> MASDYKDDDDKASDEVDAGTMANVSKKVSWSGRDRDDEEAAPLLRRTARPGGGTPLLNGAGPGAARQSPRSALFRVGHMSSVELDDELLDPDMDPPHPFPKEIPHNEKLLSLKYESLDYDNSENQLFLEEERRINHTAFRTVEIKRWVICALIGILTGLVACFIDIVVENLAGLKYRVIKGNIDKFTEKGGLSFSLLLWATLNAAFVLVGSVIVAFIEPVAAGSGIPQIKCFLNGVKIPHVVRLKTLVIKVSGVILSVVGGLAVGKEGPMIHSGSVIAAGISQGRSTSLKRDFKIFEYFRRDTEKRDFVSAGAAAGVSAAFGAPVGGVLFSLEEGASFWNQFLTWRIFFASMISTFTLNFVLSIYHGNMWDLSSPGLINFGRFDSEKMAYTIH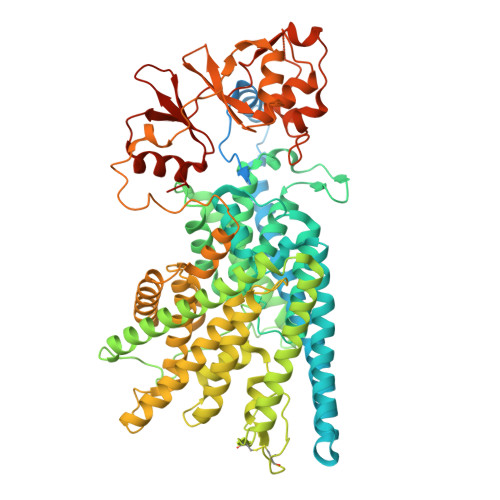EIPVFIAMGVVGGVLGAVFNALNYWLTMFRIRYIHRPCLQVIEAVLVAAVTATVAFVLIYSSRDCQPLQGGSMSYPLQLFCADGEYNSMAAAFFNTPEKSVVSLFHDPPGSYNPLTLGLFTLVYFFLACWTYGLTVSAGVFIPSLLIGAAWGRLFGISLSYLTGAAIWADPGKYALMGAAAQLGGIVRMTLSLTVIMMEATSNVTYGFPIMLVLMTAKIVGDVFIEGLYDMHIQLQSVPFLHWEAPVTSHSLTAREVMSTPVTCLRRREKVGVIVDVLSDTASNHNGFPVVEHADDTQPARLQGLILRSQLIVLLKHKVFVERSNLGLVQRRLRLKDFRDAYPRFPPIQSIHVSQDERECTMDLSEFMNPSPYTVPQEASLPRVFKLFRALGLRHLVVVDNRNQVVGLVTRKDLARYRLGKRGLEELSLAQT>MERLRQIASQATAASAAPARPAHPLDPLSTAEIKAATNTVKSYFAGKKISFNTVTLREPARKAYIQWKEQGGPLPPRLAYYVILEAGKPGVKEGLVDLASLSVIETRALETVQPILTVEDLCSTEEVIRNDPAVIEQCVLSGIPANEMHKVYCDPWTIGYDERWGTGKRLQQALVYYRSDEDDSQYSHPLDFCPIVDTEEKKVIFIDIPNRRRKVSKHKHANFYPKHMIEKVGAMRPEAPPINVTQPEGVSFKMTGNVMEWSNFKFHIGFNYREGIVLSDVSYNDHGNVRPIFHRISLSEMIVPYGSPEFPHQRKHALDIGEYGAGYMTNPLSLGCDCKGVIHYLDAHFSDRAGDPITVKNAVCIHEEDDGLLFKHSDFRDNFATSLVTRATKLVVSQIFTAANYEYCLYWVFMQDGAIRLDIRLTGILNTYILGDDEEAGPWGTRVYPNVNAHNHQHLFSLRIDPRIDG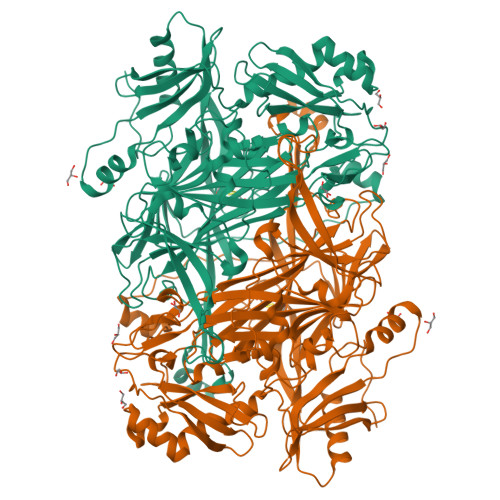DGNSAAACDAKSSPYPLGSPENMYGNAFYSEKTTFKTVKDSLTNYESATGRSWDIFNPNKVNPYSGKPPSYKLVSTQCPPLLAKEGSLVAKRAPWASHSVNVVPYKDNRLYPSGDHVPQWSGDGVRGMREWIGDGSENIDNTDILFFHTFGITHFPAPEDFPLMPAEPITLMLRPRHFFTENPGLDIQPSYAMTTSEAKRAVHKETKDKTSRLAFEGSCCGK[3x]>[2x]GGMGQTLLDALNVRVVGSGERVLVLAHGFG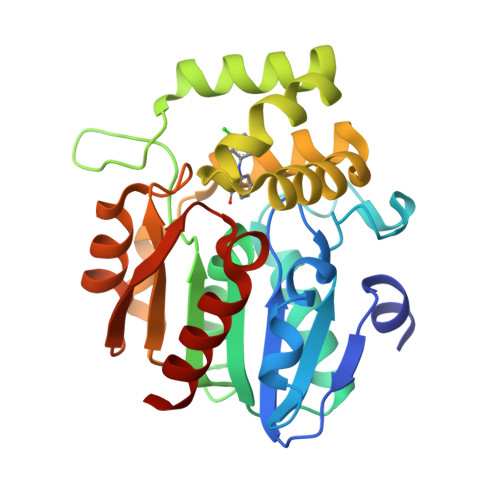TDQSAWNRILPFFLRDYRVVLYDLVCAGSVNPDFFDFRRYTTLDPYVDDLLHILDALGIDQCAYVGHSVSAMIGILASIRRPELFSKLILIGASPRFLNDEDYHGGFEQGEIEKVFSAMEANYEAWVNGFAPLAVGADVPAAVREFSRTLFNMRPDITLFVSRTVFNSDMRGVLGLVKVPCHIFQTARDHSVPASVATYLKNHLGGKNTVHWLNIEGHLPHLSAPTLLAQELRRALSHR>[4x]SNAMKIKKESLEMRQMRKKVVLIGTGLIGGSLALAIKKDHDVTITGYDIFQEQVERAKELHVVDEIAVDLQHACEEAHLIVFASPVEETKKLLHKLASFHLREDVIVTDVGSTKGSIMNEAEALFSKEISFIGGHPMAGSHKTGVESAKAHLFENAFYILTPMHHVPNEHVEELKDWLKGTGSHFLVLNTEEHDYVTGIVSHFPHLIAAGLVKQVEKHAGDNPLIHQLAAGGFK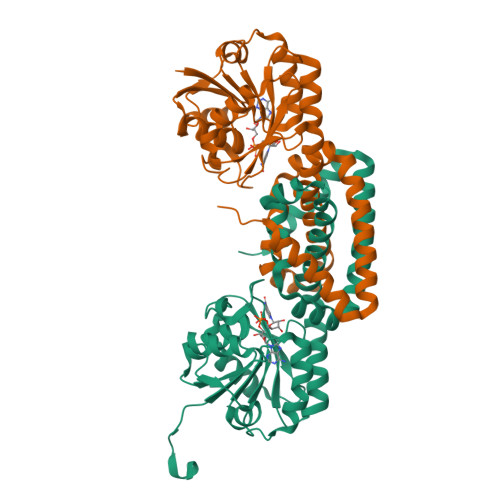DITRIASSSPKMWSDIVKQNREHLMVLLKEWISEMEDLYDTVSSGDAGEIQNYFADAKEYRDSLPVRKRGAIPAY>[2x]AAEYAVVLKTLSNPFWVDMKKGIEDEAKTLG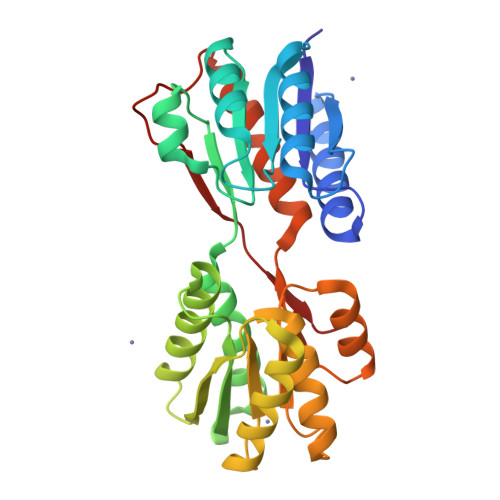VSVDIFASPSEGDFQSQLQLFEDLSNKNYKGIAFAPLSSVNLVMPVARAWKKGIYLVNLDEKIDMDNLKKAGGNVEAFVTTDNVAVGAKGASFIIDKLGAEGGEVAIIEGKAGNASGEARRNGATEAFKKASQIKLVASQPADWDRIKALDVATNVLQRNPNIKAIYCANDTMAMGVAQAVANAGKTGKVLVVGTDGIPEARKMVEAGQMTATVAQNPADIGATGLKLMVDAEKSGKVIPLDKAPEFKLVDSILVTQ>MAHHHHHHS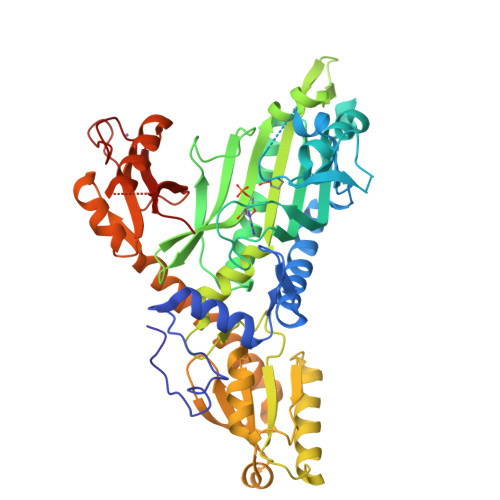KENESLLGITADKITSFADWYSQVIVKSEMIEYYDISGCYILRPWSYFIWETIQSVFDQKIKQHDVQNAYFPIFVTQKKLETEKDHVEGFSPEVAWVTKSGKSDLAEPIAIRPTSETIMYPYFAKWIRSHRDLPLKINQWTSIVRWEFKHPTPFIRTREFLWQEGHTAHSTRKEALEMVDIILNEYASIYEDLLATPVVKGTKSENEKFPGGDITKSIEGFIPEIGRAVQAATSHLLGQNFSKMFGVEFEDEKGNKEYAHQTSWGLTTRAIGVMIMTHGDNKGLVLPPKVAPVQVIIIPIIFKTVITEEQKKICNEVECILKKAGVRVKIDDRSNYTPGWKYNHWEVKGVCLRFEVGPRDIEKRSVRVVVRDNMEKMDIPISELESKIPKLLEEFQNRLLFKAKQRQNESIIRVDTFDKVMDTLNQKKMVIAPWCEDVSCEEEIKKETARLSLDNEDNQSMTGAMKSLCIPNDQIFKIEEGKTKCFFCDKLAKKFTLFGRSY[2x]> SLMALSRGLPRELAEAVAGGRVLVVGAGGIGCELLKNLVLTGFSHIDLIDLDTIDVSNLNRQFLFQKKHVGRSKAQVAKESVLQFYPKANIVAYHDSIMNPDYNVEFFRQFILVMNALDNRAARNHVNRMCLAADVPLIESGTAGYLGQVTTIKKGVTECYECHPKPTQRTFPGCTIRNTPSEPIHCIVWAKYLFNQLFGEEDADQEVSPDRADPEAAWEPTEAEARARACNEDGDIKRISTKEWAKSTGYDPVKLFTKLFKDDIRYLLTMDKLWRKRKPPVPLDWAEVQSQGEETNASDQQNEPQLGLKDQQVLDVKSYARLFSKSIETLRVHLAEKGDGAELIWDKDDPS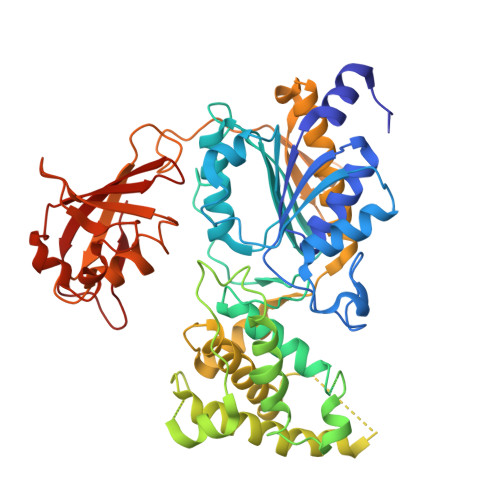AMDFVTSAANLRMHIFSMNMKSRFDIKSMAGNIIPAIATTNAVIAGLIVLEGLKILSGKIDQCRTIFLNKQPNPRKKLLVPCALDPPNPNCYVCASKPEVTVRLNVHKVTVLTLQDKIVKEKFAMVAPDVQIEDGKGTILISSEEGETEANNHKKLSEFGIRNGSRLQADDFLQDYTLLINILHSEDLGKDVEFEVVGD> NIDEYIGFDG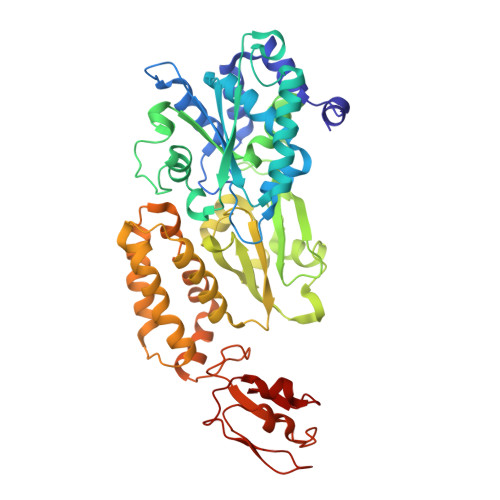YLALEKVLLTMSPVDVINEVKASGLRGRGGGGFPTGLKWQFAHDAVSEDGIKYVACNADEGDPGAFMDRSVLEGDPHAVIEAMAIAGYAVGASKGYVYVRAEYPIAVNRLQIAIDQAKEYGILGENIFETDFSFDLEIRLGAGAFVCGEETALMNSIEGKRGEPRPRPPFPANKGLFGKPTVLNNVETYANIPKIILNGAEWFASVGTEKSKGTKVFALGGKINNTGLLEIPMGTTLREIIYEIGGGIPNGKAFKAAQTGGPSGGCLPESLLDTEIDYDNLIAAGSMMGSGGLIVMDEDNCMVDVARFFLDFTQDESCGKCPPCRIGTKRMLEILERICDGKGVEGDIERLEELAVGIKSSALCGLGQTAPNPVLSTIRFFRDEYEAHIRDKKCPAGVCKHLLDFKINADTCKGCGICAKKCPADAISGEKKKPYNIDTSKCIKCGACIEACPFGSISKA>VSPPPPIADEPLTVNTGIYLIECYSLDDKAETFKVNAFLSLSWKDRRLAFDPVRSGVRVKTYEPEAIWIPEIRFVNVENARDADVVDISVSPDGTVQYLERFSARVLSPLDFRRYPFDSQTLHIYLIVRSVDTRNIVLAVDLEKVGKNDDVFLTGWDIESFTAVVKPA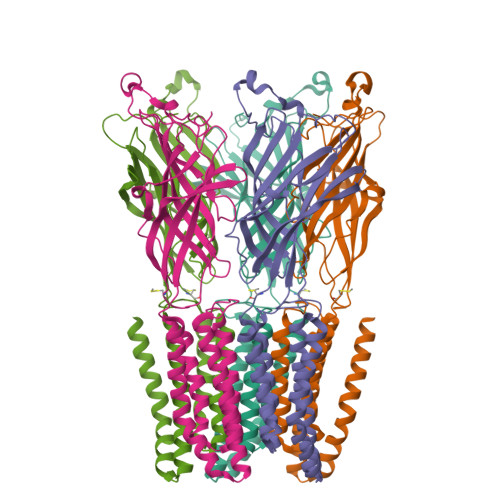NFALEDRLESKLDYQLRISRCYFSYIPNIILPMLFILFISWTAFWSTSYEANVTLVVSTLIAHIAFNILVETNLPKTPYMTYTGAIIFMIYLFYFVAVIEVTVQHYLKVESQPARAASITRASRIAFPVVFLLANIILAFLFF[5x]The A2HBD has elevated expression in F. prausnitzii A2-165 and is crucial for the transformation of acetoacetyl-CoA to 3-hydroxybutyryl-CoA in the butyrate cycle. The monomeric structure of A2HBD consists of two domains, N-terminal and C-terminal, with cofactor binding occurring at the N-terminal domain, while the C-terminal domain facilitates dimerization. The A2HBD protein exists as a hexamer in solution.

The crystal structure of the tertiary complex of A2HBD was solved at 2.2 Å resolution. The tertiary complex belonged to P3212 space group with unit cell parameters a = 90 Å, b = 90 Å, c = 212 Å and α = 90 Å, β = 90, γ = 120 Å. Notably, the tertiary-A2HBD protein manifested as a trimer, wherein only one subunit harbored acetoacetyl-CoA and NAD+. The acetoacetyl-CoA substrate is located between the clamp-roof domain (moving-helix) and clamp-base domain. When superposed to the NAD+ -bound form of the enzyme with the tertiary structure, the overall conformation has been changed, displaying an RMSD of 2.202 Å. The most notable aspect of this structural change is the movement of the clamp-roof domain, which shifts approximately 6.02 Å closer to the acetoacetyl-CoA compared to its position in the NAD complex, with a rotation of 11 degrees. Interestingly, in the tertiary structure, rotations of Arg143 toward the adenine ring were observed compared to the NAD complex, allowing the acetoacetyl-CoA to be stabilized through a cation-π interaction. The acetoacetyl group is located in hydrogen bonding distance with the sidechains of Ser117 (OB), His136 (NE2), and Asn186 (ND2). The hydroxyl group of Ser117 establishes an interaction with the NAD cofactor, thus placing this residue in a bridge with both the substrate and the cofactor. Upon substrate binding, acetoacetyl-CoA is stabilized in the closed conformation through interactions with the conserved active site residues.

>[3x]AMKIGVIGAGTMGQGIAKAFAQVEGNTVALCDIKQEWAENGLAKIKKGYEKLVAKGKIPQEKADAIVAAITPGLKENLCADCDLIVEAAFEDMKVKQTTFGELDKICKPECIFASNTASLSITEIGKGLSRPLVGMHFFNPADRMKLIEVIAGCNTPAETVEKIKEISVAIGKNPVQVNEAAGFVVNRILIPMINEAAFIKMEGVSDIAGIDTAMKLGANHPMGPLELGDFIGLDICLAIMDVLYHETGDSKYRACPLIRKMVRGGNLGCKTGKGFYVYNADRTKTPVDQL(3~{S})-1-(4-chlorophenyl)-4,4-dimethyl-3-(1,2,4-triazol-1-ylmethyl)pentan-3-ol | C16 H22 Cl N3 O | 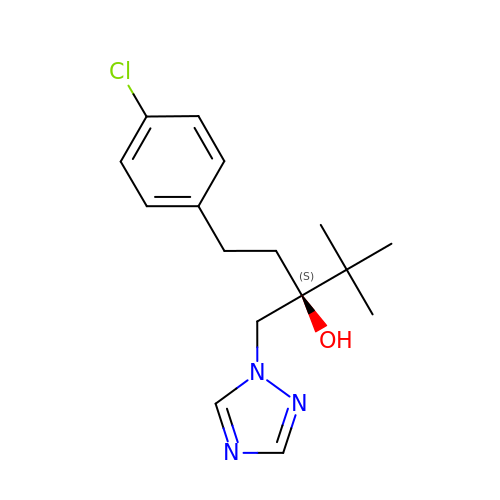PXMNMQRDXWABCY-MRXNPFEDSA-N> IPCGESCVWGPCISSAIGCSCKSKVCYRNG;> IPCGESCVWLPCISSAIGCSCKSKVCYRNG

Cyclotides are a large family of topologically unique peptides characterized by a head-to-tail cyclic backbone and three interlocked disulfide bonds. This combination of structural features forms a cyclic cystine knot (CCK) motif and confers cyclotides exceptional stability. Cyclotides are divided into three subfamilies: bracelet, Möbius, and trypsin inhibitor subfamilies. Since cyclotides were first reported two decades ago, studies on bracelet cyclotides have been hampered by their low synthetic yields because of poor oxidative folding efficiency.

To explore the effect of substituting the Ile residue in loop 2 to Gly, we first introduced the mutation into cyO2, which is considered a prototypical bracelet cyclotide and is one of the most studied. Remarkably, the point mutation of Ile to a smaller residue led to a significant improvement in folding yield from negligible amounts for cyO2 to over 50% for the mutant cyO2. We found that when the loop 2 Ile is mutated to Gly, bracelet cyclotides could be folded with high yield, albeit with loss of activity. All [I11G] mutants did not bind the model membrane at peptide concentrations up to 128 µM, except [I11G]hD, which showed an 18-fold weaker affinity to membranes compared to its parent peptide. The negative effect of the [I11G] bracelet cyclotide mutation on lipid binding was expected, as the mutation reduces surface hydrophobicity, a previously reported determinant of membrane binding. [I11L] mutants exhibited similar or slightly higher cytotoxicity compared to their parent cyclotides, whereas the [I11G] mutants had substantially reduced or no activity, which correlates well with their membrane binding. Having determined the crystal structures of wild-type cyO2 and hyen D, we were interested in definitively showing their Ile-11 to Gly and Leu mutants have native-like structures to support our earlier NMR chemical shift analysis. Their structures were solved using racemic or quasi-racemic crystallography. Like the case of cyO2 mutants, [I11L]hD and [I11G]hD structures only exhibited minor differences in the mainchain and sidechain conformations, confirming both Leu and Gly substitutions are well tolerated by the bracelet fold.> MHDANIRVAIAGAGGRMGRQLIQAALALEGVQLGAALEREGSSLLGSDAGELAGAGKTGVTVQSSLDAVKDDFDVFIDFTRPEGTLNHLAFCRQHGKGMVIGTTGFDEAGKQAIRDAAADIAIVFAANFSVGVNVMLKLLEKAAKVMGDYTDIEIIEAHHRHKVDAPSGTALAMGEAIAHALDKDLKDCAVYSREGHTGERVPGTIGFATVRAGDIV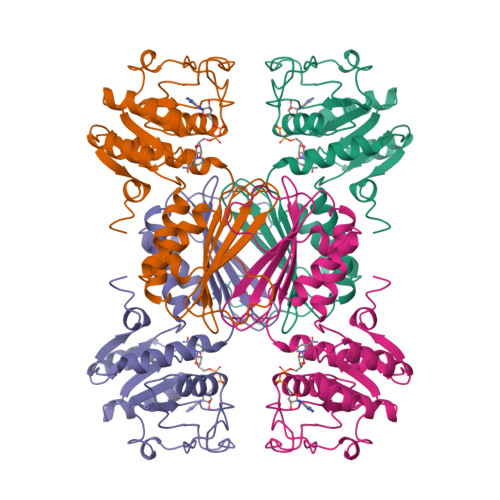GEHTAMFADIGERLEITHKASSRMTFANGAVRSALWLSGKESGLFDMRDVLDLNNL> MTVTRRHFLKLSAGAAVAGAFTGLGLSLAPTVARAELQKLQWAKQTTSICCYCAVGCGLIVHTAKDGQGRAVNVEGDPDHPINEGSLCPKGASIFQLGENDQRGTQPLYRAPFSDTWKPVTWDFALTEIAKRIKKTRDASFTEKNAAGDLVNRTEAIASFGSAAMDNEECWAYGNILRSLGLVYIEHQARIUHSPTVPALAESFGRGAMTNHWNDLANSDCILIMGSNAAENHPIAFKWVLRAKDKGATLIHVDPRFTRTSARCDVYAPIRSGADIPFLGGLIKYILDNKLYFTDYVREYTNASLIVGEKFSFKDGLFSGYDAANKKYDKSMWAFELDANGVPKRDPALKHPRCVINLLKKHYERYNLDKVAAITGTSKEQLQQVYKAYAATGKPDKAGTIMYAMGWTQHSVGVQ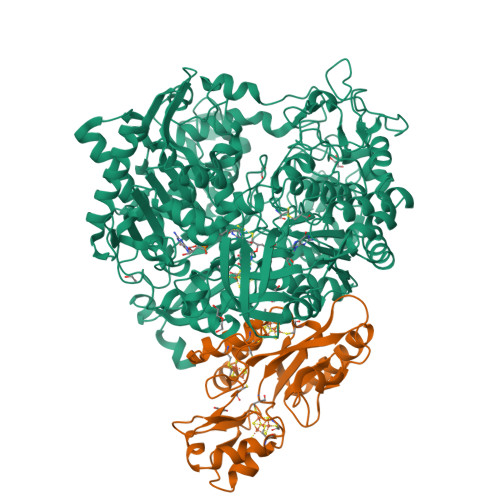NIRAMAMIQLLLGNIGVAGGGVNALRGESNVQGSTDQGLLAHIWPGYNPVPNSKAATLELYNAATPQSKDPMSVNWWQNRPKYVASYLKALYPDEEPAAAYDYLPRIDAGRKLTDYFWLNIFEKMDKGEFKGLFAWGMNPACGGANANKNRKAMGKLEWLVNVNLFENETSSFWKGPGMNPAEIGTEVFFLPCCVSIEKEGSVANSGRWMQWRYRGPKPYAETKPDGDIMLDMFKKVRELYAKEGGAYPAPIAKLNIADWEEHNEFSPTKVAKLMNGYFLKDTEVGGKQFKKGQQVPSFAFLTADGSTCSGNWLHAGSFTDAGNLMARRDKTQTPEQARIGLFPNWSFCWPVNRRILYNRASVDKTGKPWNPAKAVIEWKDGKWVGDVVDGGGDPGTKHPFIMQTHGFGALYGPGREEGPFPEHYEPLECPVSKNPFSKQLHNPVAFQIEGEKKAVCDPRYPFIGTTYRVTEHWQTGLMTRRCAWLVEAEPQIFCEISKELAKLRGIGNGDTVKVSSLRGALEAVAIVTERIRPFKIEGVDVHMVGLPWHYGWMVPKNGGDTANLLTPSAGDPNTGIPETKAFMVDVRKVWSHPQFEK;> MGKMFFVDLSRCTACRGCQIACKQWKNLPAEETRNTGSHQNPPDLSYVTLKTVRFTEKSRKGPGIDWLFFPEQCRHCVEPPCKGQADVDLEGAVVKDETTGAVLFTELTAKVDGESVRSACPYDIPRIDPVTKRLSKCDMCNDRVQNGLLPACVKTCPTGTMNFGDEQEMLALAEKRLAEVKKTYPGAVLGDPNDVRVVYLFTRDPKDFYEHAVADLAPSMMTRQQLFARLFRPRA tert-butyl (3R)-1,2,3,4-tetrahydroquinolin-3-ylcarbamate | C14 H20 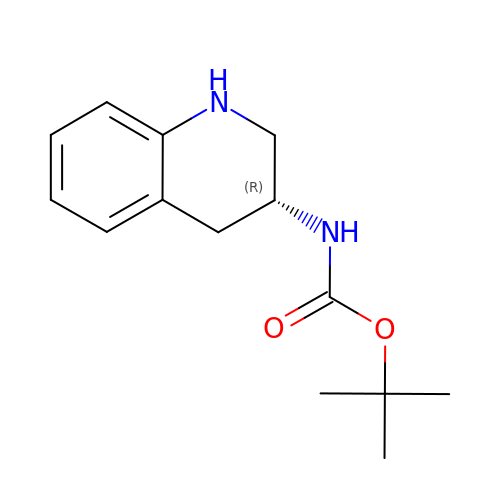N2 O2 | GAURNOYXRZQBNV-LLVKDONJSA-N>SIVSKSIVNADAEARYLSPGELERIKTFVVGGDRRLRIAQTIAESRERIVKQAGNQLFQKRPDVVSPGGNAYGEDMTATCL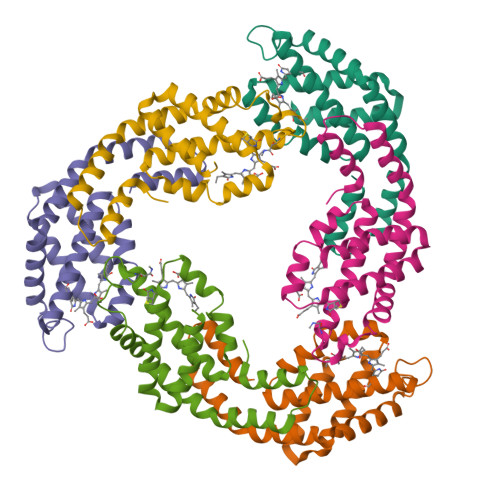RDLDYYLRLVTYGVVSGDITPIEEIGIVGVREMYKSLGTPIEAVAEGVRELKSAATALLTGEDADEAGAYFDYVIGALS[3x];>MQDAITAVINASDVQGKYLDSSALDRLKSYFQSGELRVRAAATISANSALIVKEAVAKSLLYSDITRPGGNMYTTRRYAACIRDLEYYLRYATYAMLAGDTSILDERVLNGLKETYNSLGVPIGATVQAIQAIKEVTASLVGPDAGREMGVYLDYISSGLS[3x]> MEERNDWHFNIGAMYEIENVEGYGEDMDGLAEPSVYFNAANGPWRIALAYYQEGPVDYSAGKRGTWFDRPELEVHYQFLENDDFSFGLTGGFRNYGYHYVDEPGKDTANMQRWKIAPDWDVKLTDDLRFNGWLSMYKFANDLNTTGYADTRVETETGLQYTF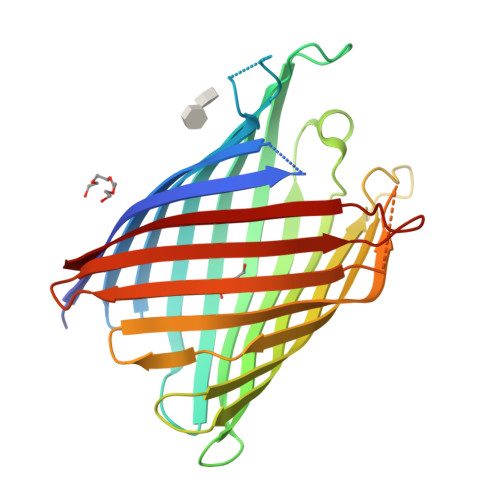NETVALRVNYYLERGFNMDDSRNNGEFSTQEIRAYLPLTLGNHSVTPYTRIGLDRWSNWDWQDDIEREGHDFNRVGLFYGYDFQNGLSVSLEYAFEWQDHDEGDSDKFHYAGVGVNYSF> GSSK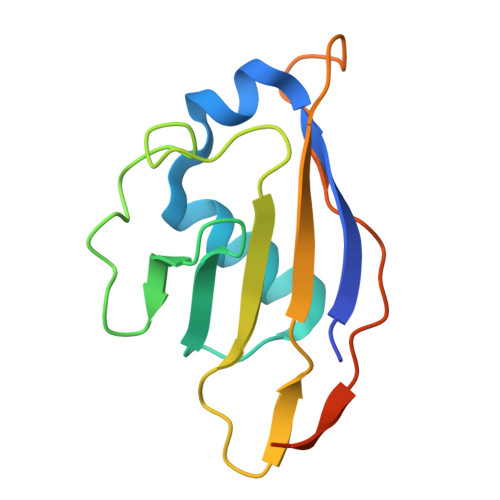VCRGVIKLSSDCLNKMKLSDFVVLIREKYSYPQDISLLDASNQRLLFDYDFEDLNDRTLSEINLGNGSIILFSDEEGDTMIRKAIELFLDVDDELPCNTCSLPDVEVPLIKANNSPSKNEEEE> MPVAGSELPRRPLPPAAQERDAEPRPPHGELQYLGQIQHILRCGVRKDDRTGTGTLSVFGMQARYSLRDEFPLLTTKRVFWKGVLEELLWFIKGSTNAKELSSKGVKIWDANGSRDFLDSLGFSTREEGDLGPVYGFQWRHFGAEYRDMESDYSGQGVDQLQRVIDTIKTNPDDRRIIMCAWNPRDLPLMALPPCHALCQFYVVNSELSCQLYQRSGDMGLGVPFNIASYALLTYMIAHITGLKPGDFIHTLGDAHIYLNHIEPLKIQLQREPRPFPKLRILRKVEKID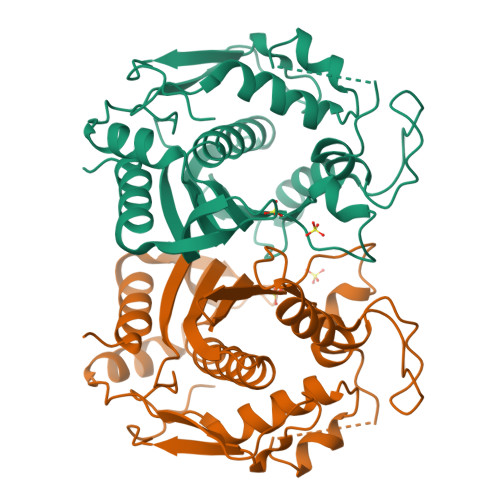DFKAEDFQIEGYNPHPTIKMEMAVHHHHH>[2x]GMFAGSIPMYIRVVSITAQSKLQFDMTVTYFENVWSP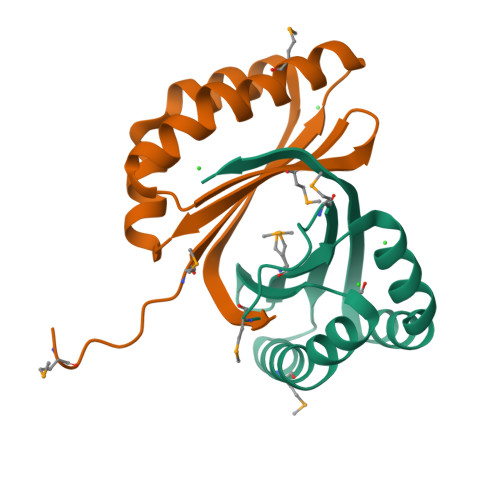KVISLGAISAEFVQSNENSGMYIIHYPDKQTAISVFDKIKPEVDEVRTQNRIQITEGKRLFRVD>GSARPKLRVVTLVEHPFVFTRESDEDGQCPAGQLCLDPGTNDSARLDALFAALVNGSVPRTLRRCCYGYCIDLLERLAEDLAFDFELYIVGDGKYGALRDGRWTGLVGDLLAGRAHMAVTSFSINSARSQVVDFTSPFFSTSLGIMVRTRGTELSGIHDPKLHHPSQGFRFGTVWESSAEAYIKASFPEMHAHMRRHSAPTTPHGVAMLTSDPPKLNAFIMDKSLLDYEVSIDADCKLLTVGKPFAIEGYGIGLPQNSPLTSNLSEFISR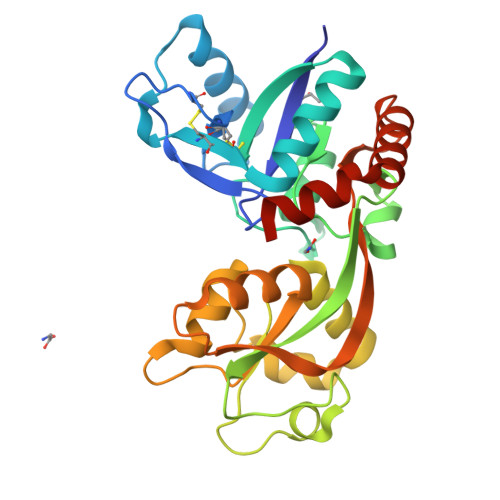YKSSGFIDLLHDKWYKMVPCGK[2x]> MGSSHHHHHHSQDPDQPGNSSLENLPPVAASIEQLLERQWSEGQQFLLEQGTPSDILG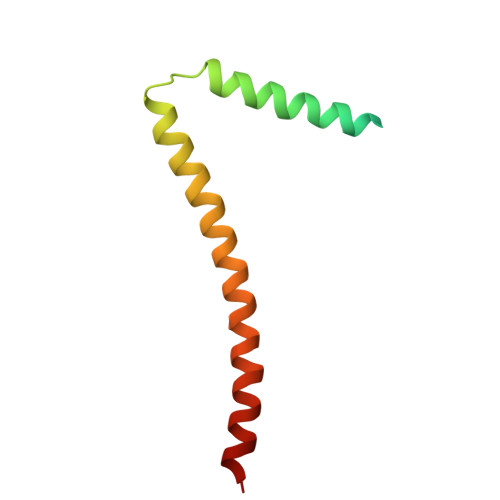MLKSLHQLQVENRRLEEQIKNLTAKKERLQLLNAQLSVPF> PPSVFAEVPQAQPVLVFKLTADFREDPDPRKVNLGVGAYRTDDCHPWVLPVVKKVEQKIANDNSLNHEYLPILGLAEFRSCASRLALGDDSPA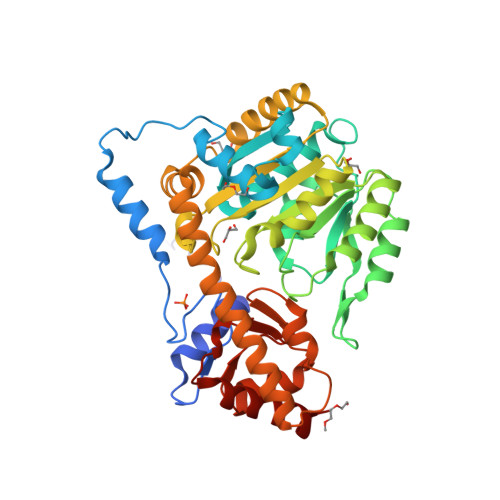LKEKRVGGVQSLGGAGALRIGADFLARWYNGTNNKNTPVYVSSPTWENHNAVFSAAGFKDIRSYRYWDAEKRGLDLQGFLNDLENAPEFSIVVLHACAHNPTGIDPTPEQWKQIASVMKHRFLFPFFDSAYQGFASGNLERDAWAIRYFVSEGFEFFCAQAFSKNFGLYNERVGNLTVVGKEPESILQVLSQMEKIVRITWSNPPAQGARIVASTLSNPELFEEWTGNVKTMADRILTMRSELRARLEALKTPGTWIHITDQIGMFSFTGLNPKQVEYLVNEKHIYLLPSGRINVSGLTTKNLDYVATSIHEAVTKIQ>MNVASRVVVNADRVKGTINRNIYGHFSEHLGRCIYEGLWVGEDSPIPNTNGIRNDVLEALKQMKIPVLHWPGGCFADEYHWKDGVGPREKRKRMVNTHWGGVIENNHFGTHEFMMLCELLGCEPYISGNVGSGTVQEMSEWVEYITFDGESPMANWRRENGREKPWRIKYWGVGNENWGCGGNMRAEYYADLYRQFQTYLRNYGDNKLHKIACGANTADYHWTEVLMKQAAPFMHGLSLHYYTVPGPWEKKGPATGFTTDEWWVTLKKALFMDELVTKHSAIMDVYDPDKRIDLIVDEWGTWYDVEPGTNPGFLYQQ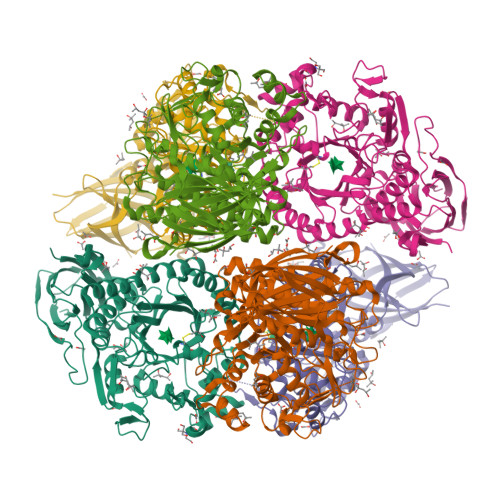NSIRDALVAGATLHIFHRHCDRVRMANIAQLVNVMQSVILTEGERMLLTPTYHVFNMFKVHQDAELLDTWESVERTGPEGELPKVSVSASRAADGKIHISLCNLDFETGASVDIELRGLNGGVSATGTTLTSGRIDGHNTFDEPERVKPAPFRDFKLEGGHLNASLPPMSVTVLELTAG[3x]>CSSLSIRTTDDKSLFARTMDFTMEPDSKVIIVPRNYGIRLLEKENVVINNSYAFVGMGSTDITSPVLYDGVNEKGLMGAMLYYATFATYADEPKKGTTGINPVYVISQVLGNCVTVDDVIEKLTSYTLLNEANIILGFAPPLHYTFTDASGESIVIEPDKTGITIHRKTIGVMTNSPGYEWHQTNLRAYIGVTPNPPQDIMMGDLDLTPFGQGAGGLGLPGDFTPSARFLRVAYWKKYTEKAKNETEGVTNLFHILSSVNIPKGVVLTNEGKTDYTIYTSAMCAQSKNYY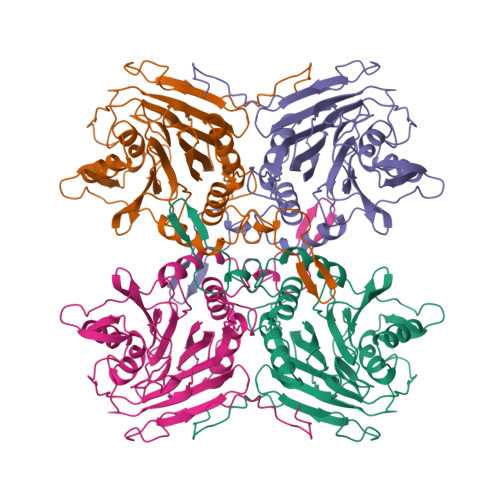FKLYDNSRISAVSLMAENLNSQDLITFEWDRKQDIKQLNQVNVMS[8x]>[4x]MSVVI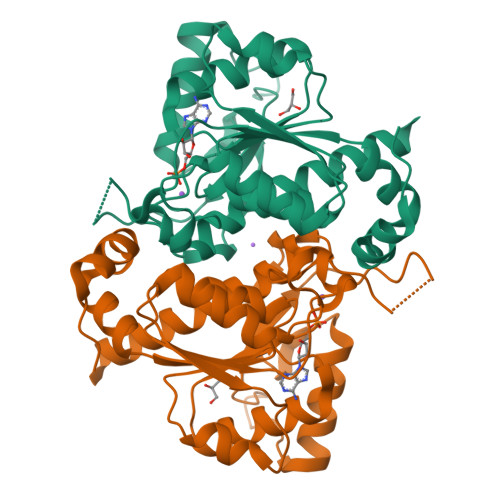SDAWRQRFGGTARLYGEKALQLFADAHICVVGIGGVGSWAAEALARTGIGAITLIDMDDVCVTNTNRQIHALRDNVGLAKAEVMAERIRQINPECRVTVVDDFVTPDNVAQYMSVGYSYVIDAIDSVRPKAALIAYCRRNKIPLVTTGGAGGQIDPTQIQVTDLAKTIQDPLAAKLRERLKSDFGVVKNSKGKLGVDCVFSTEALVYPQSDGTVCAMKATAEGPKRMDCASGFGAATMVTATFGFVAVSHALKKMMAKAARQG> AGVDEAAIRATEQAGGEWLSHGRTYAEQRFSPLKQIDASNVRSLGLAWYMDLDNTRGLEATPLFHDGVIYTSMSWSRVIAVDAASGKELWRYDPEVAKVKARTSCCDAVNRGVALWGDKVYVGTLDGRLIALDAKTGKAIWSQQTTDPAKPYSITGAPRVVKGKVIIGNGGAEYGVRGFVSAYDADTGKLAWRFYTVPGDPALPYEHPELREAAKTWQGDQYWKLG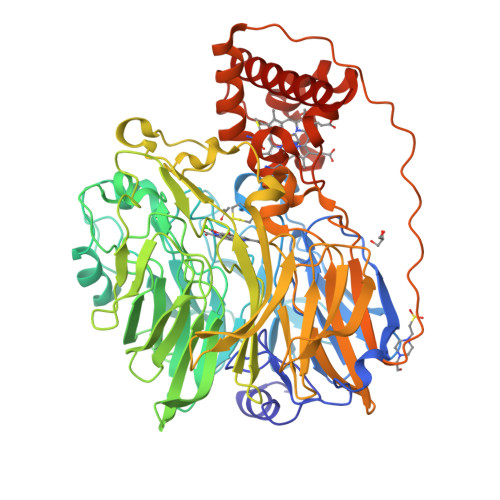GGGTVWDSMAYDPELDLLYVGTGNGSPWNREVRSPGGGDNLYLSSILAIRPDTGKLAWHYQVTPGDSWDFTATQQITLAELNIDGKPRKVLMQAPKNGFFYVLDRTNGKLISAEKFGKVTWAEKVDLATGRPVEAPGVRYEKEPIVMWPSPFGAHNWHSMSFNPGTGLVYIPYQEVPGVYRNEGKDFVTRKAFNTAAGFADATDVPAAVVSGALLAWDPVKQKAAWKVPYPTHWNGGTLSTAGNLVFQGTAAGQMHAYSADKGEALWQFEAQSGIVAAPMTFELAGRQYVAIMAGWGGVATLTGGESMNLPGMKNRSRLLVFALDGKAQLPPPAPAPAKVERVPQPVTAAPEQVQAGKQLYGQFCSVCHGMGTISGGLIPDLRQSSDATREHFQQIVLQGALKPLGMPSFDDSLKPEEVEQIKLYVMSREYEDYMARHKAAP(1S,5S,6R)-10-[(3,5-dichlorophenyl)sulfonyl]-5-[(1R)-1,2-dihydroxyethyl]-3-[2-(3,4-dimethoxyphenoxy)ethyl]-3,10-diazabicyclo[4.3.1]decan-2-one | C26 H32 Cl2 N2 O8 S | 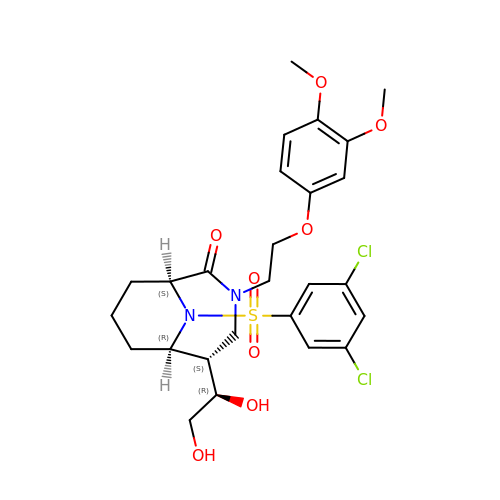JKYLGBPUGDRSCP-BJESRGMDSA-N> GSEQLGELMEPALGYVVKVPVSSFENKKVDISDIEVITNGNLDDVPYKANSSKYNYPDIKTKDSSLQYVRSGYVIDGEHSGSNEKGYVYYKGNSPAKELPVNQLLTYTGSWDFTSNANLNNEEGRPNYLNDDYYTKAIGKRVGLVSGDAKPAKHKYTSQFEVDFATKKMTGKLSDKEKTIYT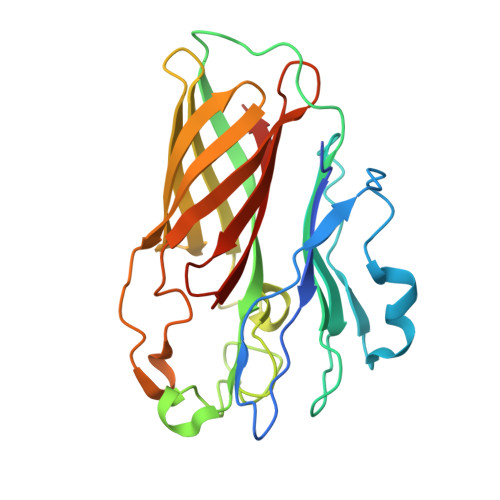VNADIRGNRFTGAATASDKNKGKGESYNFFSADSQSLEGGFYGPKAEEMAGKFVANDKSLFAVFSAKHNGSNV> MASHHHHHHSGMDQTPIRVLLAKVGLDGHDRGVKVVARALRDAGMDVIYSGLHRTPEEVVNTAIQEDVDVLGVSLLSGVQLTVFPKIFKLLDERGAGDLIVIAGGVMPDEDAAAIRKLGVREVLLQDTPPQAIIDSIRS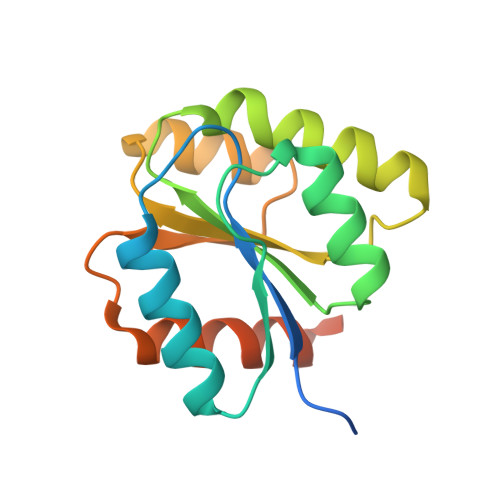LVAARGARGSAWSHPQFEK> AQSVPYGISQIKAPA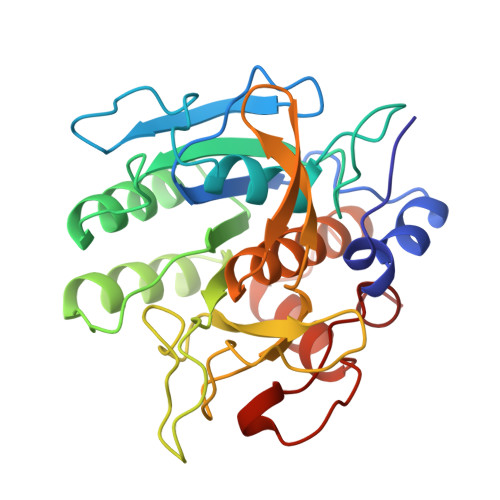LHSQGYTGSNVKVAVIDSGIDSSHPDLNVRGGASFVPSETNPYQDGSSHGTHVAGTIAALNNSIGVLGVSPSASLYAVKVLDSTGSGQYSWIINGIEWAISNNMDVINMSLGGPTGSTALKTVVDKAVSSGIVVAAAAGNEGSSGSTSTVGYPAKYPSTIAVGAVNSSNQRASFSSAGSELDVMAPGVSIQSTLPGGTYGAYNGTCMATPHVAGAAALILSKHPTWTNAQVRDRLESTATYLGNSFYYGKGLINVQAAAQ> ATSDDWKSKAIYQLLTDRFGRADDSTSNCSNLSNYCGGTYEGITKHLDYISGMGFDAIWISPIPKNSDGGYHGYWATDFY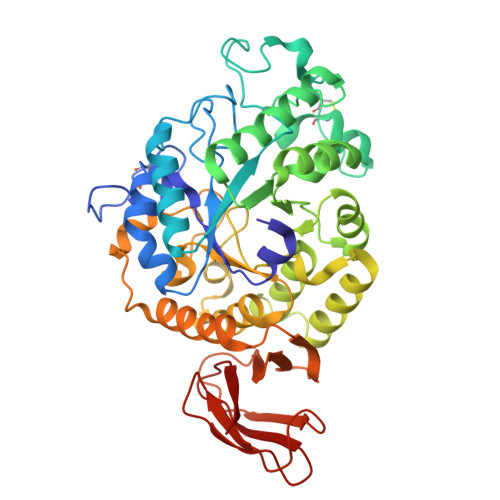QLNSNFGDESQLKALIQAAHERDMYVMLDVVANHAGPTSNGYSGYTFGDASLYHPKCTIDYNDQTSIEQCWVADELPDIDTENSDNVAILNDIVSGWVGNYSFDGIRIDTVKHIRKDFWTGYAEAAGVFATGEVFNGDPAYVGPYQKYLPSLINYPMYYALNDVFVSKSKGFSRISEMLGSNRNAFEDTSVLTTFVDNHDNPRFLNSQSDKALFKNALTYVLLGEGIPIVYYGSEQGFSGGADPANREVLWTTNYDTSSDLYQFIKTVNSVRMKSNKAVYMDIYVGDNAYAFKHGDALVVLNNYGSGSTNQVSFSVSGKFDSGASLMDIVSNITTTVSSDGTVTFNLKDGLPAIFTSA>[2x]GMATLGANASLYSEQHRITYYECDRTGRATLTTLIDIAVLASEDQSDALGLTTEMVQSHGVGWVVTQYAIDITRMPRQDEVVTIAVRGSAYNPYFAYREFWIRDADGQQLAYITSIWVMMSQTTRRIVKILPELVAPYQSEVVKRIPRLPRPI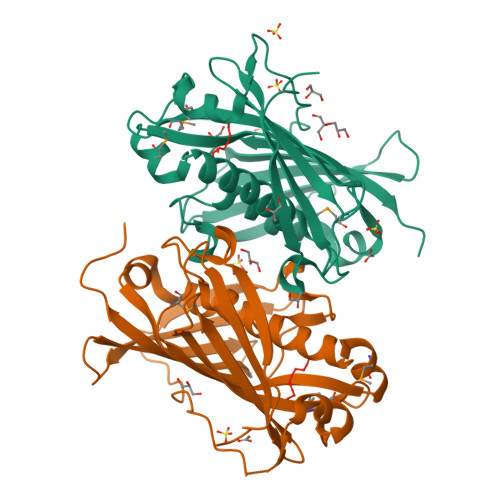SFEATDTTITKPYHVRFFDIDPNRHVNNAHYFDWLVDTLPATFLLQHDLVHVDVRYENEVKYGQTVTAHANILPSEVADQVTTSHLIEVDDEKCCEVTIQWRTLPEPIQ>MDSTEAEQMDTEQATNQTAEAGGGGGGGGGGGGGGGGVGNSTGGFNNTTEFKVINNEVYITCHATRMVHINQADTDEYLIFNAGRTTDTKTHQQKLNLEFFVYDDFHQQVMTPWYIVDSNAWGVWMSPKDFQQMKTLCSEISLVTLEQEIDNVTIKTVTETNQGNASTKQFNNDLTASLQVALDTNNILPYTPAAPLGETLGFVPWRATKPTQYRYYHPCYIYNRYPNIQKVATETLTWDAVQDDYLSVDEQYFNFITIENNIPINILRTGDNFHTGLYEFNSKPCKLTLSYQSTRCLGLPPLCKPKTDTTHKVTSKENGADLIYIQGQDNTRLGHFWGEERGKKNAEMNRIRPYNIGYQYPEWIIPAGLQGSYFAGGPRQWSDTTKGAGTHSQHLQQNFSTRYIYDRNHGGDNEVDLLDGIPIHERSNYYSDNEIEQHTAKQPKLRTPPIHHSKIDSWEEEGWPAASGTHFEDEVIYLDYFNFSGEQELNFPHEVLDDAAQMKKLLNSYQPTVAQDNVGPVYPWGQIWDKKPHMDHKPSMNNNAPFVCKNNPPGQLFVKLTENLTDTFNYDENPDRIKTYGYFTWRGKLVLKGKLSQVTCWNPVKRELIGEPGVFTKDKYHKQIPNNKGN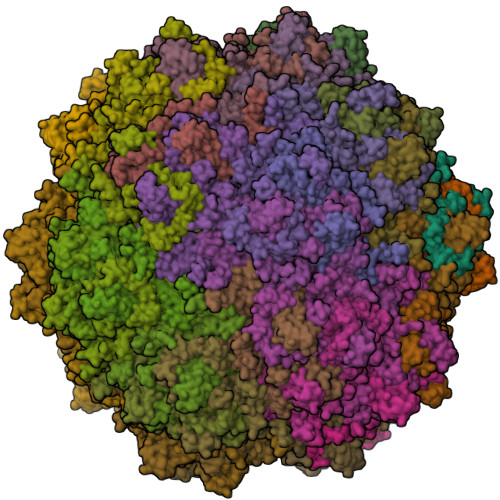FEIGLQYGRSTIKYIY[60x]(Z)-3-(4-chlorophenyl)-2-mercaptoacrylic acid 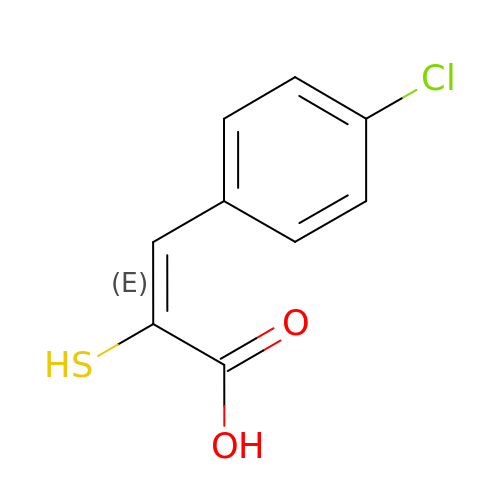| C9 H7 Cl O2 S | VYZXSVKKNPHGGV-VMPITWQZSA-N> SLSDKDKAAVRALWSKIGKSSDAIGNDALSRMIVVYPQTKIYFSHWPDVTPGSPNIKAHGKKVMGGIALAVSKIDDLKTGLMELSEQHAYKLRVDPSNFKILNHCILVVISTMFPKEFTPEAHVSLDKFLSGVALALAERYR;> VEWTDKERSIISDIFSHMDYDDIGPKALSRCLVVYPWTQRYFSGFGNLYNAEGIMSNANVAAHGIKVLHGLDRGMKNMDNIADAYTDLSTLHSEKLHVDPDNFKLLSDCITIVLAAKMGHAFTAETQGAFQKFLAAVVSAL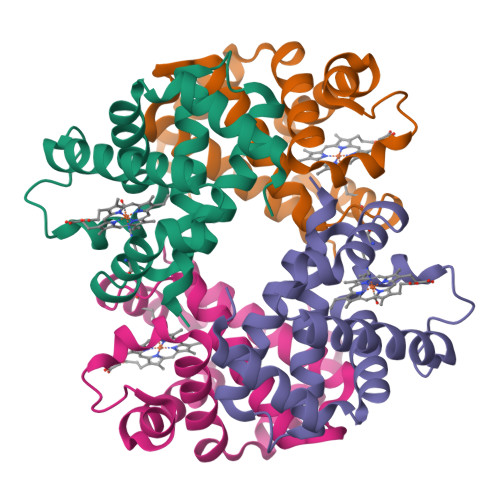GKQYH>[8x]MHHHHHHHHHHSSGVDLGTENLYFQSNATIELSIVIPMYNEEDNLEHLFARLLEVLTPL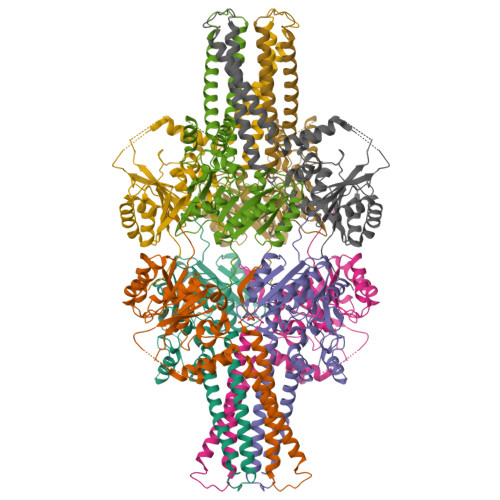KITYEIICVNDGSKDKTLKQLIDCYQSNRQIKIVNLSRNFGKEIALSAGIDYAQGNAVIPIDADLQDPPELIHELVDKWREGYDIVYATRRSRQGETWVKQFTAKMFYKVIGRMTEIKIPPNTGDFRLMDRKVVNAIKQLPERTRFMKGLFAWVGYRQTFVLFDREPRFQGQTKWNYWKLWNFALDGIFSFSLLPLKVWTYLGSIISLLSLAYASFLILKTITLGVDVPGYASLMVAILFLGGVQLISLGVIGEYLGRVYEEVKARPLYLVSDLWGLEYLPLEKLN>[2x]MSTQYETQGYTINNAGRRLVVDPITRIQGHMRCEVNINDQNVITNAVSCGTMFRGLEIILQGRDPRDAWAFVERICGVCTGVHALASVYAIEDAIGIKVPDNANIIRNIMLATLWCHDHLVHFYQLAGMDWIDVLDALKADPRKTSELAQSLSSWPKSSPGYFFDVQNRLKKFVEGGQLGIFRNGYWGHPQYKLPPEANLMGFAHYLEALDFQREIVKIHAVFGGKNPHPNWIVGGMPCAINIDESGAVGAVNMERLNLVQSIITRTADFINNVMIPDALAIGQFNKPWSEI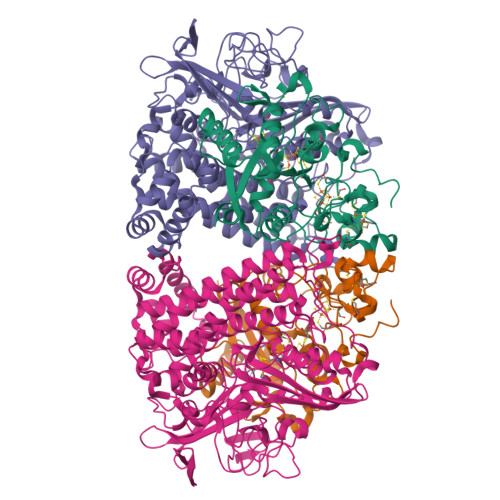GTGLSDKCVLSYGAFPDIANDFGEKSLLMPGGAVINGDFNNVLPVDLVDPQQVQEFVDHAWYRYPNDQVGRHPFDGITDPWYNPGDVKGSDTNIQQLNEQERYSWIKAPRWRGNAMEVGPLARTLIAYHKGDAATVESVDRMMSALNLPLSGIQSTLGRILCRAHEAQWAAGKLQYFFDKLMTNLKNGNLATASTEKWEPATWPTECRGVGFTEAPRGALGHWAAIRDGKIDLYQCVVPTTWNASPRDPKGQIGAYEAALMNTKMAIPEQPLEILRTLHSFDPCLACSTH;>[2x]LENKPRIPVVWIHGLECTCCTESFIRSAHPLAKDVILSLISLDYDDTLMAAAGTQAEEVFEDIITQYNGKYILAVEGNPPLGEQGMFCISSGRPFIEKLKRAAAGASAIIAWGTCASWGCVQAARPNPTQATPIDKVITDKPIIKVPGCPPIPDVMSAIITYMVTFDRLPDVDRMGRPLMFYGQRIHDKCYRRAHFDAGEFVQSWDDDAARKGYCLYKMGCKGPTTYNACSSTRWNDGVSFPIQSGHGCLGCAENGFWDRGSFYSRVVDIPQMGTHSTADTVGLTALGVVAAAVGVHAVASAVDQRRRHNQQPTETEHQPGNEDKQA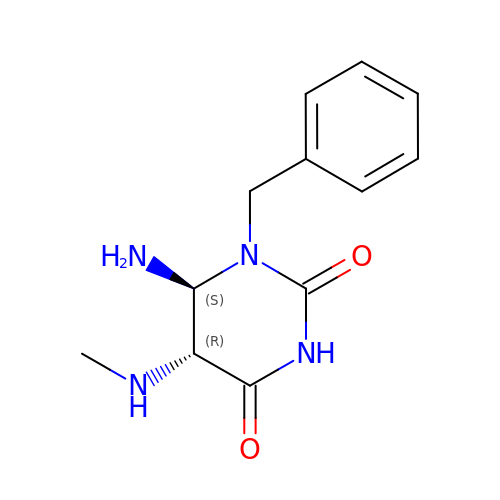6-amino-1-benzyl-5-(methylamino)pyrimidine-2,4(1H,3H)-dione | C12 H16 N4 O2 | ROGMXQYZAWKCLY-ZJUUUORDSA-N> GHMRSMVSKGEELIKENMRMKVVMEGSVNGHQFKCTGEGEGNPYMGTQTMRIKVIEGGPLPFAFDILATSFLYGSRTFIKYPKGIPDFFKQSFPEGFTWERVTRYEDGGVVTVMQDTSLEDGCLVYHVQVRGVDFPSNGPVMQKKTKGWEPITEMMYPADGGLRGYTHMALKVDGGGHLSCSFVTTYRSKKTVGNIKMPGIHAVDH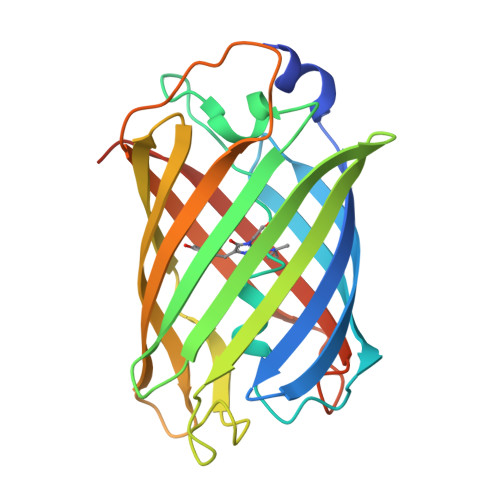RLERLEESDNEMFVVLREHSVAKFAGRGGMDELYK> MADLAESNIKVMCRFRPLNESEVNRGDKYIAKFQGEDTVVIASKPYAFDRVFQSSTSQEQVYNDAAKKIVKDVLEGYNGTIFAYGQTSSGKTHTMEGKLHDPEGMGIIPRIVQDIFNYIYSMDENLEFHIKVSYFEIYLDKIRDLLDVSKTNLSVHEDKNRVPYVKGATERFVSSPDEVMDTIDEGKSNRHVAVTNMNEHSSRSHSIFLI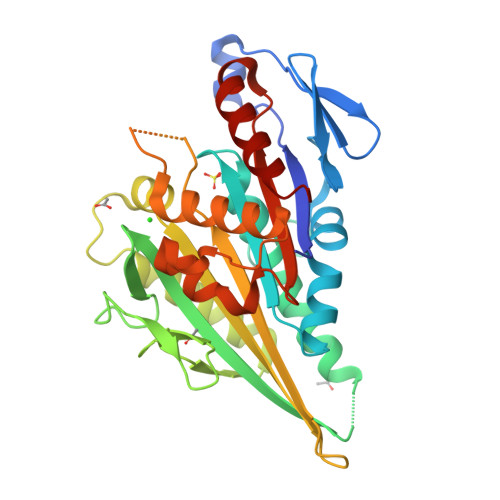NVKQENTQTEQKLSGKLYLVDLAGSEKVSKTGAEGAVLDEAKNINKSLSALGNVISALAEGSTYVPYRDSKMTRILQDSLGGNARTTIVICCSPSSYNESETKSTLLFGQRAKTI> MSETFTKGMARNIYFGGSVFFILLFLALTYHTEKTLPERTNEAAMSAAVVRGKLVWEQNNCVGCHTLLGEGAYFAPELGNVVGRRGGEEGFNTFLQAWMKIQPLNVPGRRAMPQFHLSEGQVDDLAEFLKW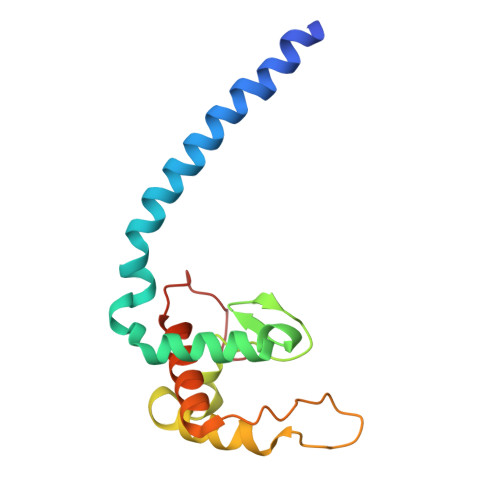SSKIDTNQWPPNKEG>[4x]MQIPASEQETLVRPKPLLLKLLKSVGAQ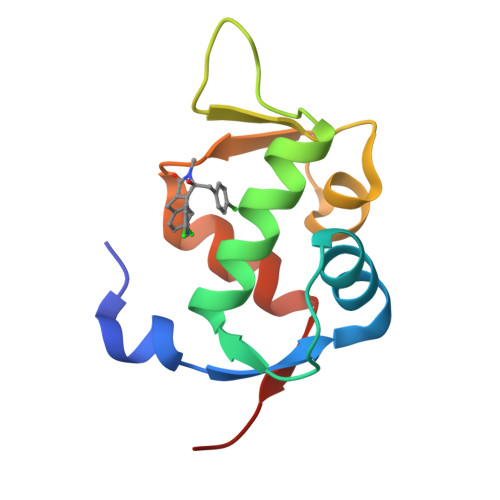KDTYTMKEVLFYLGQYIMTKRLYDEKQQHIVYCSNDLLGDLFGVPSFSVKEHRKIYTMIYRNLVVVNQQ>[2x]MKIKAISIDIDGTITYPNRMIHEKALEAIRRAESLGIPIMLVTGNTVQFAEA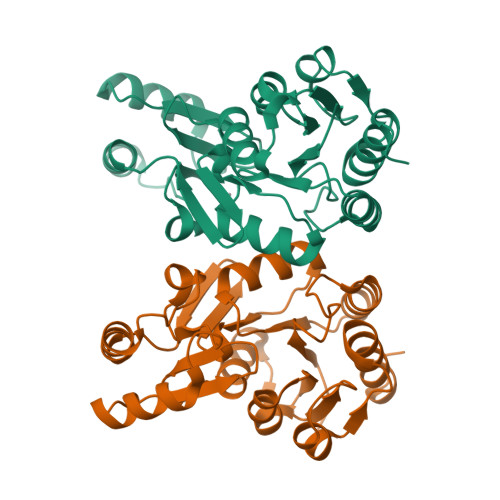ASILIGTSGPVVAEDGGAISYKKKRIFLASMDEEWILWNEIRKRFPNARTSYTMPDRRAGLVIMRETINVETVREIINELNLNLVAVDSGFAIHVKKPWINKGSGIEKASEFLGIKPKEVAHVGDGENDLDAFKVVGYKVAVAQAPKILKENADYVTKKEYGEGGAEAIYHILEKFGYL> MEQRITLKDYAMRFGQTKTAKDLGVYPSSINQAIHAG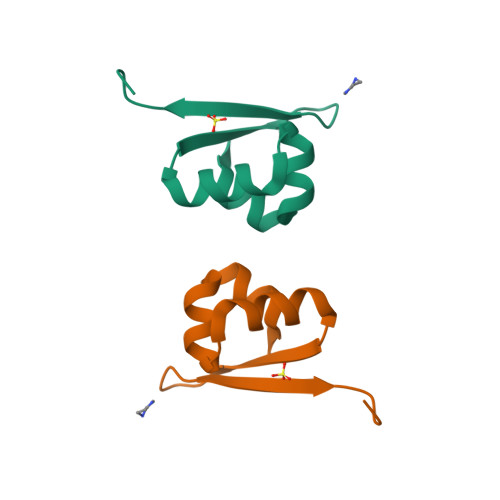RKIFLTINADGSVYAEEVKPFPSNKKTTA> DAP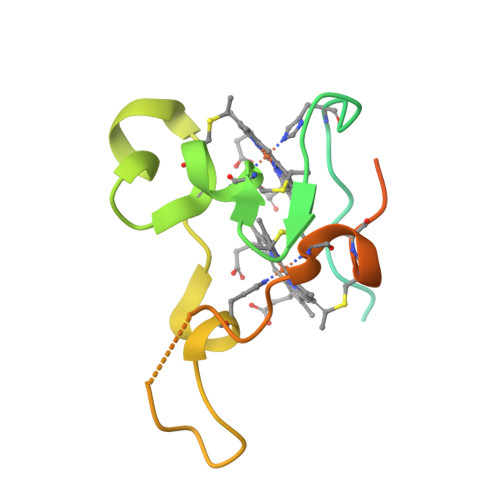AVGKDLTQAAENIPPAFHNAPRQGELPALNYVNQPPMVPHSVANYQVTKNVNQCLNCHSPENSRLSGATRISPTHFMDRDGKVGSSSSPRRYFCLQCHVSQANVDPIVPNDFKPMKGYGN> MATQEEILDAALVSGDSSQLTDSHLVALRLQQQVERIRQTRTQLLDGLYQNLSQAYDPGAASMWVLPANPDNTLPFLIGDKGRVLASLSLEAGGRGLAYGTNVLTQLSGTNAAHAPLLKRAVQWLVNGDPGAATAKDFKVSVVGVDKTAALNGLKSAGLQPADAACNALTDASCASTSKLLVLGNGASAASLSATVRARLQAGLPILFVHTNGWNQSSTGQQILAGLGLQEGPYGGNYWDKDRVPSSRTRTRSVELGGAYGQDPALVQQIVDGSWRTDYDWSKCTSYVGRTTCDDVPGLSDFSKRVDVLKGALDAYNQKAQNLFALPGTTSLRLWLLWADAVRQNIRYPMDKAADTARFQETFVADAIVGYVREAGAAQKELGSYAGQRQQSMPVSGSEETLTLTLPSAQGFTAIGRMAAPGKRLSIRIEDAGQASLAVGLNTQRIGSTRLWNTRQYDRPRFLKSPDIKLQANQSVALVSPYGGLLQLVYSGATPGQTVTVKVTGAASQPFLDIQPGEDSSQAIADFIQALDADKADWLEIRSGSVEVHAKV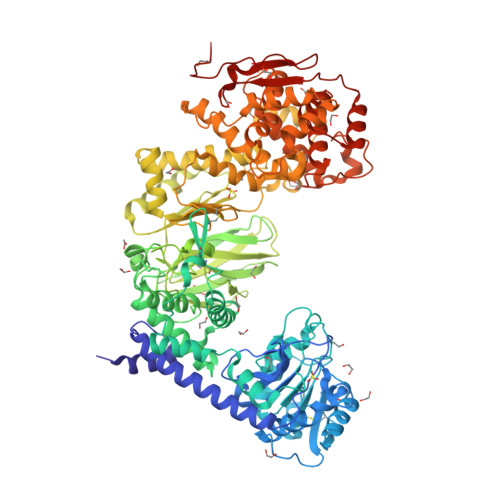EKVRGSIDKDYGGDVQRFIRELNEVFIDDAYTLAGFAIPNQAKTPAIQQECAARGWDCDSETLHKLPGTQHINVDQYAQCGGGCSGNPYDQTWGLNPRGWGESHELGHNLQVNRLKVYGGRSGEISNQIFPLHKDWRVLREFGQNLDDTRVNYRNAYNLIVAGRAEADPLAGVNKRLWEDPGTYALNGERMAFYTQWVHYWADLKNDPLQGWDIWTLLYLHQRQVDKSDWDANKAALGYGTYAQRPGNSGDASSTDGNDNLLLGLSWLTQRDQRPTFALWGIRTSAAAQAQVAAYGFAEQPAFFYANNRTNEYSTVKLLDMSQGSPAWPFPLEHHHHHH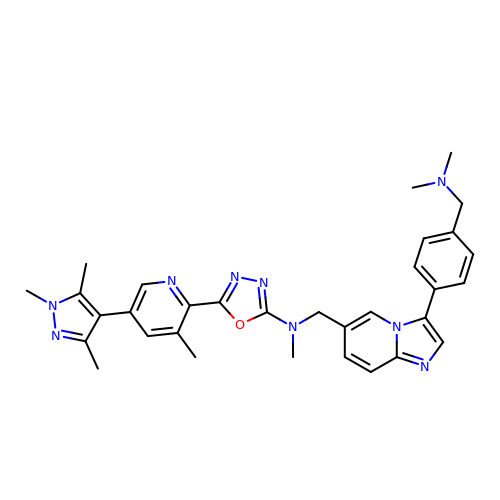~{N}-[[3-[4-[(dimethylamino)methyl]phenyl]imidazo[1,2-a]pyridin-6-yl]methyl]-~{N}-methyl-5-[3-methyl-5-(1,3,5-trimethylpyrazol-4-yl)pyridin-2-yl]-1,3,4-oxadiazol-2-amine | C32 H35 N9 O | CZIXXCVLEHVEBZ-UHFFFAOYSA-N6-methyl-5-[3-methyl-3-(3,4,5-trimethoxyphenyl)but-1-yn-1-yl]pyrimidine-2,4-diamine | C19 H24 N4 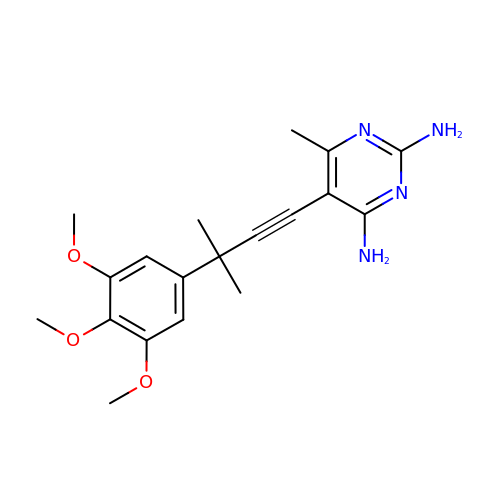O3 | FJNFXXGWYVMQNA-UHFFFAOYSA-N> VQIHDITGKDCQDIANKGAKQSGLYFIKPLKANQQFLVYCEIDGSGNGWTVFQKRLDGSVDFKKNWIQYKEGFGHLSPTGTTEFWLGNEKIHLISTQSAIPYALRVELEDWNGRTSTADYAMFKVGPEADKYRLTYAYFAGGDAGDAFDGFDFGDDPSDKFFTSHNGMQFSTWDNDNDKFEGNCAEQDGSGWWMNKCHAGHLNGVYYQGGTYSKASTPNGYDNGIIWATWKTRWYSMKKTTMKIIPF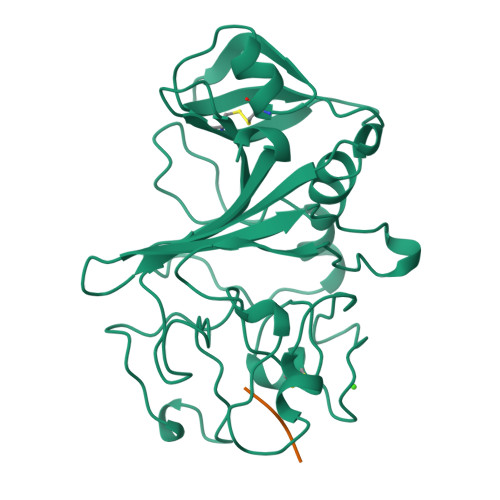NRLTIGEGQQHHLGGAKQAGDV;> GPRP>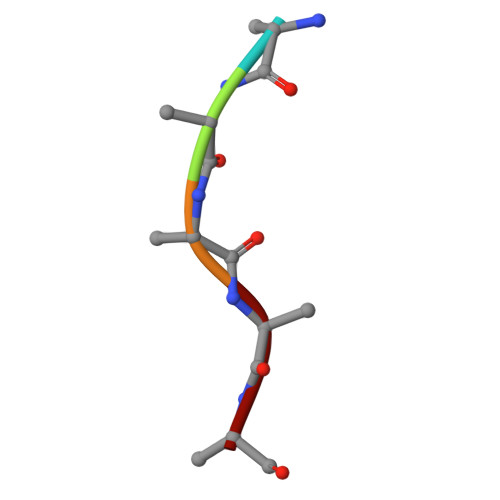 AAAAA>[2x]MAIFSVYVVNKAGGLIYQLDSYAPR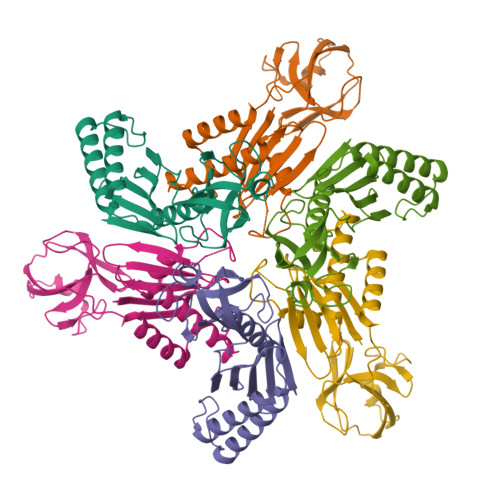AEAEKTFSYPLDLLLKLHDERVLVAFGQRDGIRVGHAVLAINGMDVNGRYTADGKEVLEYLGNPANYPVSIRFGRPRLTSNEKLMLASMFHSLFAIGSQLSPEQGSSGIEMLETDTFKLHCYQTLTGIKFVVLADPRQAGIDSLLRKIYEIYSDFALKNPFYSLEMPIRCELFDQNLKLALEVAEKAGTFGPGSLEHHHHHH>TRKVAIYGKGGIG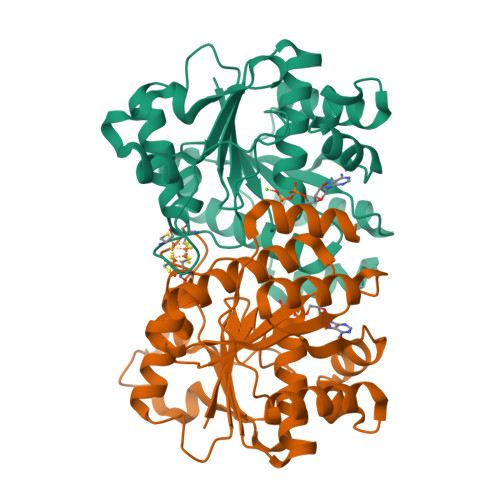KSTTTQNTAAALAYFHDKKVFIHGCDPKADSTRLILGGKPQETLMDMLRDKGAEKITNDDVIKKGFLDIQCVESGGPEPGVGCAGRGVITAIDLMEENGAYTDDLDFVFFDVLGDVVCGGFAMPIRDGKAQEVYIVASGEMMAIYAANNICKGLVKYAKQSGVRLGGIICNSRKVDGEREFLEEFTAAIGTKMIHFVPRDNIVQKAEFNKKTVTEFAPEENQAKEYGELARKIIENDEFVIPKPLTMDQLEDMVVKYGIAD[4x]> YPQSIDWRAKGAVTPVKNQGACGSCWAFSTIATVEGINKIVTGNLLELSEQELVDCDKHSYGCKGGYQTTSLQYVANNGVHTSKVYPYQAKQYKCRATDKPGPKVKITGYKRVPSNCETSFLGALANQPLSVLVEAGGKPFQLYKSGVFDGPCGTKLDHAVTAVGYGTSDGKNYIIIKNSWGPNWGEKGYMRLKRQSGNSQGTCGVYKSS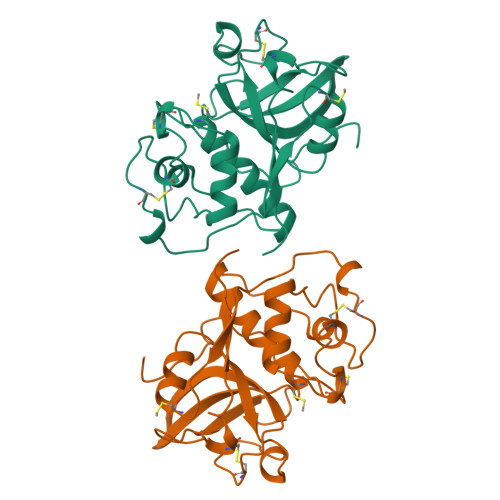YYPFKGFA> KNIESLFDYSAGQFEFIDHLLTMGVGVHFAALIFFL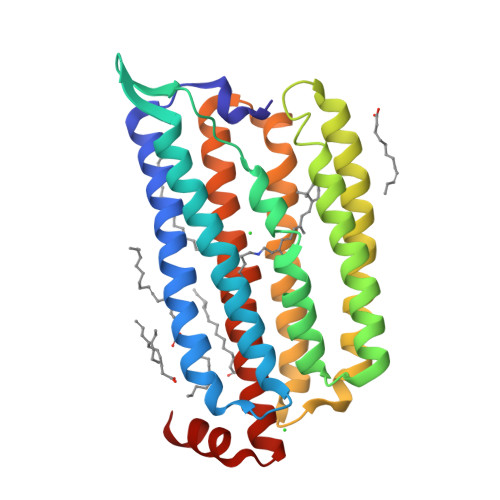VVSQFVAPKYRIATALSCIVMVSAGLILNSQAVMWTDAYAYVDGSYQLQDLTFSNGYRYVNWMATIPCLLLQLLIVLNLKGKELFSTATWLILAAWGMIITGYVGQLYEVDDIAQLMIWGAVSTAFFVVMNWIVGTKIFKNRATMLGGTDSTITKVFWLMMFAWTLYPIAYLVPAFMNNADGVVLRQLLFTIADISSKVIYGLMITYIAIQQSAAAGYVPAQQALGRI Unlike the dissociated systems of individual enzymes that make up type II FAS systems in plants and bacteria, Type I FAS systems in fungi and animals are large complexes that integrate the key enzymatic activities required for fatty acid biosynthesis. In particular, yeast type I FASs are 2.6 MDa hetero-dodecameric complexes with an α6β6 configuration, which form a cage-like structure comprising two dome-shaped reaction chambers on either side of a central platform. Along with structural support regions, enzymatic domains form the walls of the reaction chambers, with most active sites facing the chamber interior. The mobile acyl-carrier protein (ACP) domain tethers the growing fatty acid chain and carries it between active sites, so each can act on this in turn.

ACP density was weak (only becoming fully apparent when inspecting the map at a threshold of approx. 1 σ) and poorly resolved, as was also the case for previous EM density maps of S. cerevisiae FAS (e.g., EMD-10420, EMD-0178). In an attempt to improve the quality of the cryoEM density corresponding to the ACP domain, we performed focussed 3D classification within the reaction chamber of the complex. While classification with a regularisation parameter (‘T’ number) of 20 did not reveal any meaningful classes, using a higher value of 40 (i.e., putting a higher relative weighting on the experimental data than on the prior/reference) yielded a class containing relatively well resolved ACP density. Particles from this class were taken forward for asymmetric reconstruction, yielding a complete FAS map of 3.1-Å resolution. In the latter map, the additional density is consistent with the ACP domain of the α subunit of FAS, given the fit-to-density of an ACP domain homology model. Ultimately, the new density was of sufficient quality to build an atomic model of the ACP domain. Interestingly, ACP domain residue S178 (which tethers the growing fatty acid chain) is located ~ 18 Å away from the KS active site, which is in agreement with the length of the phosphopantetheine arm (18 Å). Focussed classification led to an improvement in the strength and quality of the ACP density that was sufficient to allow atomic modelling, probably as result of grouping together only subparticles with ACP domains in the same relative position (adjacent to the KS domain, as has been observed in several other yeast FAS structures) at the time of vitrification. Use of an expanded mask for focussed classification revealed classes with putative ACP density in other positions within the complex interior. These classes contained relatively few subparticles, suggesting that the vast majority of ACP domains were adjacent to the KS domain, with the remainder either missing or occupying other positions.

> MRPEVEQELSHVLLTELLAYQFASPVRWIETQDVFLKDYNTERVVEIGPSPTLAGMASRTIKAKYESYDAALSLQRQVLCYAKDTKEIYYTPDPADIAPPIKEEAETSAAATSSSAPAAAAPVSAAPAAAPSGPVAEIPDEPVKAALVLHVLVAHKLKKSLDAVPLSKAIKDLVGGKSTVQNEILGDLGKEFGSTPEKPEDTPLQELAEQFQDTFPGSLGKQTGSLVNRLMSSKMPGGFSLSVARKYLQTRWGLGPGRQDSVLLVALVNEPGARLSSDGEAKEFLDSCAQKYASGAGITLAQAAAGGAGSSGAGGAVIDAEAFEELTKDNRVLARQQLEVLARYLKYDLTKGEKSLVKEKEASSLLQQELDLWAEEHGEIYAQGIKPVFSHLKARTYDSYWNWARQDALSMYFDIIFGKLTDVDRETVSQCIQLMNRSNPTLIKFMQYHIDHCPEYKGETYQLAKSLGQQLIDNCIQVANQDPVYKDISYPTGPHTEVDSKGNIVYKEVNRKSVRKLEQYVFEMSQGGELTKEVQPTIQEDLAKIYEALNKQASTESQLEFNKLYNSLIEFVEKSKEIEVSKSINAVLASKSSDSDRSAEISSLSEKTSIVDPVSGGIPPETVPFLHLKKKLPSGEWVFDRDTSALFLDGLQKGAVNGISYKGKNVLITGAGAGSIGAEVLQGLISGGAKVIVTTSRFSKKVTEYYQDIYARFGAAGSCLIVVPFNQGSKQDVEALIDYIYRDVKDEGLGWDLDAVIPFAAIPEAGIEIDELGSKSELAHRIMLTNLLRLLGEVKKQKFTRAINTRPAQIILPLSPNHGTFGSDGLYSESKLGLETLFNRWYSESWSEQLTVCGAIIGWTRGTGLMSGNNIIAEGLEKLGVRTFSQKEMAFNILGLMTPELTEMCQNGPVVADLNGGLQFIENLREYTAQLRNEIYETSEVRRAVSIETGIETRVVNGENADAPYQKARIEPRANLKFEFPPLKSHKEIQNKAPGLEGLLDLERVIVVTGFGEVSPWGNTRTRWEMEAFGEFSIEGCLEMAWIMGFIKYHNGNLKGKPYTGWIDAKTNEPVEDKDIKKKYEEEILAHAGIRLIEPELFRGYNPEKKELIQEVIIEQDMAPFVTDESTAQQYKLQHEDAVDILKSEESDEYTVTFKKGARLFVPKALRFDRLVAGQIPTGWDAKRYGISEDTISQVDPVTLYALVSTIEALLSAGITDPYEFYKYVHVSEVGNCSGSGMGGVSALRGMFRDRYSDKPVQNDILQESFINTMSAWVNMLLLSSSGPIKTPVGACATAVESVDIGVETILSGKAKICLVGGYDDFQEEGSYEFANMNATSNSLDEFDHGRTPQEMSRPATTTRNGFMEAQGSGTQVIMNAELAIKMGVPIYAIVALTATATDKIGRSVPAPGKGILTTAREHHGSLKTKSPKLDIKYRTRQLNKRKDQIKQWVEDELEYIREEAAELANSDAKFDAVSFVSERTEEVYREATKQVKMAQQEWGNEFWKNDPRIAPLRGALATFNLTVDDLGVASFHGTSTKANDKNESITINKMMQHLGRSEGNPVFGVFQKYLTGHPKGAAGAWMLNGAIQILQTGIVPGNRNADNVDKILEDFEYVLYPSRSIQTDGIKACSVTSFGFGQKGGQAIVVHPDYLFASLDSETFEEYKTKVEARYKSTYRYMHNAIIRNTMFVAKSDPPYTDELEQPVYLDPLARVNNCKKNPSKLVFVNADVQSKQNFVGKSANDTAKVISSLTSDVTSGGKGVGVDVELISAINNENHTFIERNFTENEISYCASAPSSKSSLAGTWSAKEAVFKALGVESKGAGASLKDIEIVRDSKGAPTVVLHGDAKSAASAAGVKNVKVSISHDDVQSVAVAISEF>MASPVIYQAEDAIIYNAILETVNAGYTGSCYVNYHNEVGGYIEWNVNAPSSGSYALIFRYANGTTANRPMRITVNGNIVKPSMDFVSTGAWTTWNEAGIVANLNQGNNVIRATAIASDGGPNVDYLKVFSANAFQPVSLEHHHHHH[2x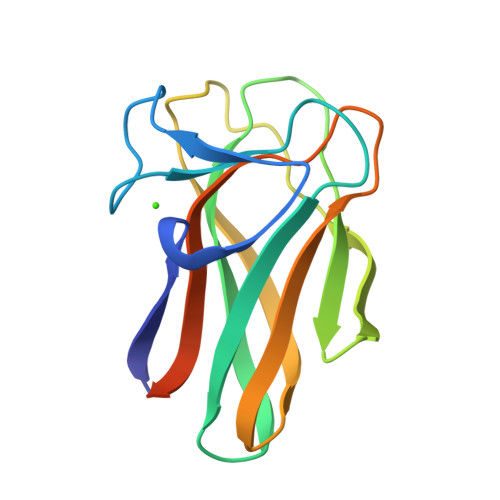]> KQLTKCALSHELNDLAGYRDITLPEWLCIIFHISGYDTQAIVKNSDHKEYGLFQINDKDFCESSTTVQSRNICDISCDKLLDDDLTDDIMCVKKILD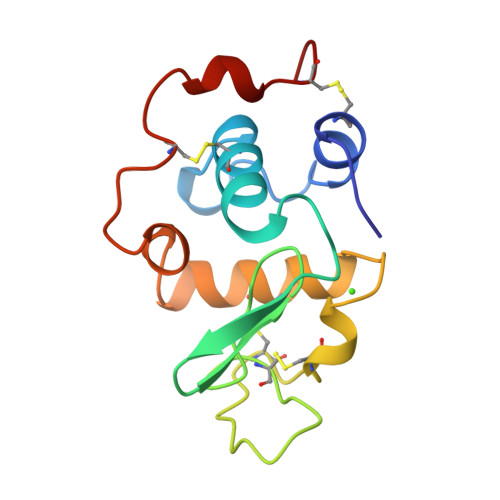IKGIDYWLAHKPLCSDKLEQWYCEAQ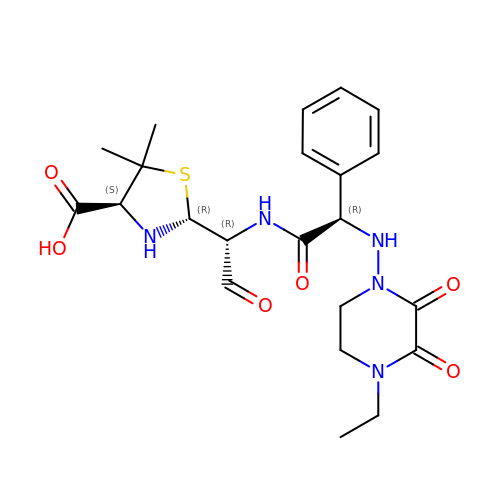(2R,4S)-2-[(1R)-1-({(2R)-2-[(4-ethyl-2,3-dioxopiperazin-1-yl)amino]-2-phenylacetyl}amino)-2-oxoethyl]-5,5-dimethyl-1,3-thiazolidine-4-carboxylic acid | C22 H29 N5 O6 S | FLMJTSOTBGMFLJ-XLMAVXFVSA-N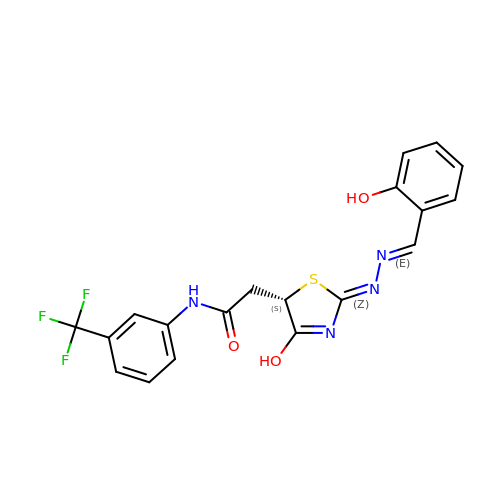2-{(2Z,5S)-4-hydroxy-2-[(2E)-(2-hydroxybenzylidene)hydrazinylidene]-2,5-dihydro-1,3-thiazol-5-yl}-N-[3-(trifluoromethyl)phenyl]acetamide | C19 H15 F3 N4 O3 S | OBVIGUGYWMTZGZ-MQEPLNOPSA-N>ATYEDLISHKHDYPKEIYKESHYIRRNTRLDVIKKIPQFEQKSKEWLKQRTESLTATAISVVFDEDPYKHPIVILLDKCGRGLPFVENKFVHHGNKYEQIGTMFYSFRNNVEVGEYGLLQHSGHKFIAASPDGICSKKANTGGLSKLVGRLLEIKFPFSREINNSGDLDGDICPHYYFLQVQTQLYVTEMDECDFLQCKIDEYDSWEDFVKDSNPIVPGLSKTTNLEKGCLIQLSDKNLIGSDDKEKCLYNSKYIYPPKLHMTNEEIAAWISSEIANYHNNDLSENYMIDAVIYWRLSQVTCNLIKLNKEAFEEKIPLLQQFWDYVLFYR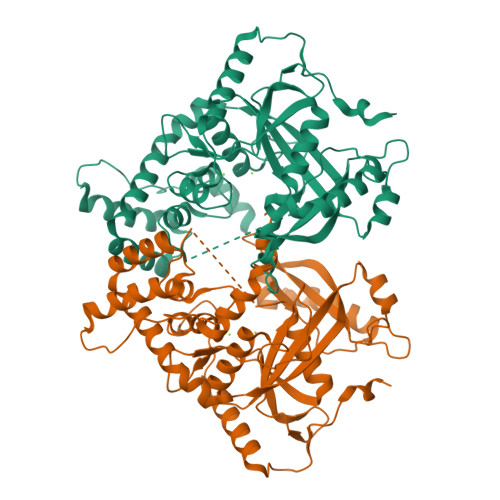QHSDKLDKLIKFVEKVKEDNSAEIFSYINEDFLSLNKDSKYEPLYQEETEWRKKYNQIKAK[2x]> GPLGSSQIPASEQETLVRPKPLLLKLLKSVGAQKDTYTMKEVLFYLGQYIMTKRLY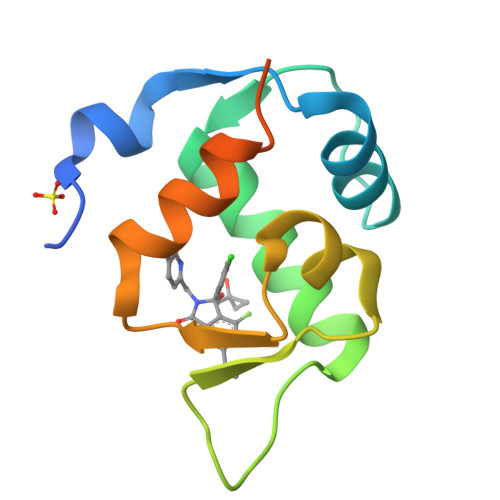DAAQQHIVYCSNDLLGDLFGVPSFSVKEHRKIYTMIYRNLVVVNQQESSDSGTSVSEN>[2x]DYKDDDDKVLGLKYEEIDCLINDEHTIKGRREGNEVFLPFTWVEKYFDVYGKVVQYDGYDRFEFSHSYSKVYAQRAPYHPDGVFMSFEGYNVEVRDRVKCISGVEGVPLSTQWGPQGYFYPIQIAQYGLSHYSKNLTEKPPHIEVYETAEDRDKNKPNDWTVPKGCFMANVADKSRFTNVKQFIAPETSEGVSLQLGNTKDFIISFDLKFLTNGSVSVVLETTEKNQLFTIHYVSNAQLIAFKERDIYYGIGPRTSWSTVTRDLVTDLRKGVGLSNTKAVKPTKIMPKKVVRLIAKGKGFLDNI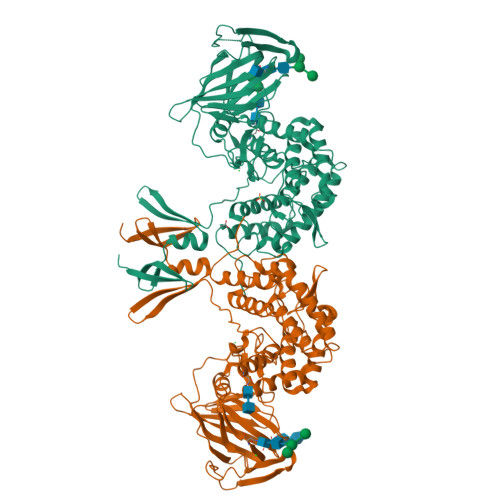TISTTAHMAAFFAASDWLVRNQDEKGGWPIMVTRKLGEGFKSLEPGWYSAMAQGQAISTLVRAYLLTKDHIFLNSALRATAPYKFLSEQHGVKAVFMNKHDWYEEYPTTPSSFVLNGFMYSLIGLYDLKETAGEKLGKEARSLYERGMESLKAMLPLYDTGSGTIYDLRHFMLGIAPNLARWDYHTTHINQLQLLSTIDESPVFKEFVKRWKSYLKGSRAKHN> SGISLDNSYKMDYPEMGLCIIINNKNF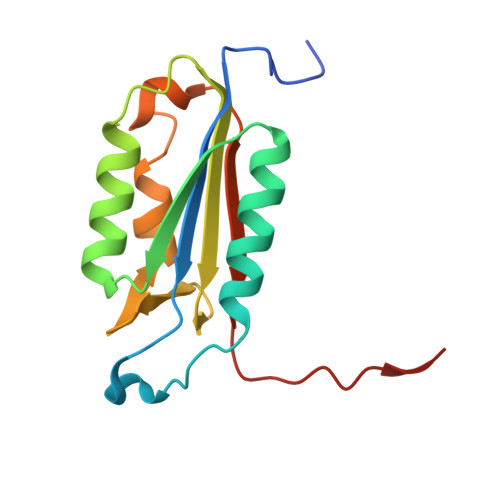HKSTGMTSRSGTDVDAANLRETFRNLKYEVRNKNDLTREEIVELMRDVSKEDHSKRSSFVCVLLSHGEEGIIFGTNGPVDLKKITNFFRGDRCRSLTGKPKLFIIQACRGTEFDCGIETD>[4x]MSYQSTIVPV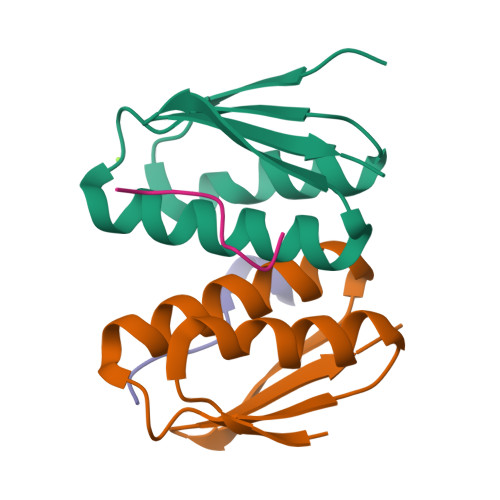ELHSFEDAQVIGGAFRDGDAVVFDMSLLSREEARRIVDFAAGLCFALRGKMQKIDSVTFAVVPE;>[4x]DDLDVPSFLQ> GGUUAUUCAGAUUAGGUAGUCGAAUGACC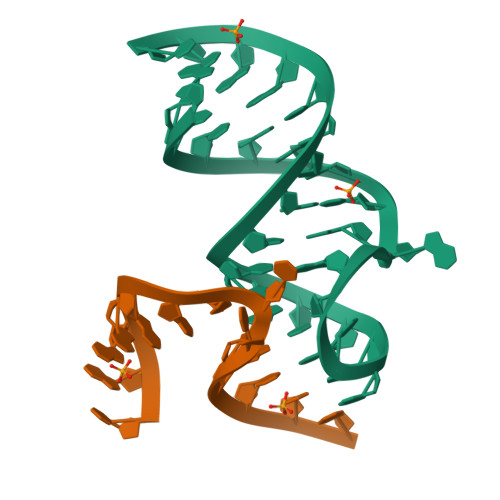;> UAAGAAAUUUACCU3,5,3'TRIIODOTHYRONINE | C15 H12 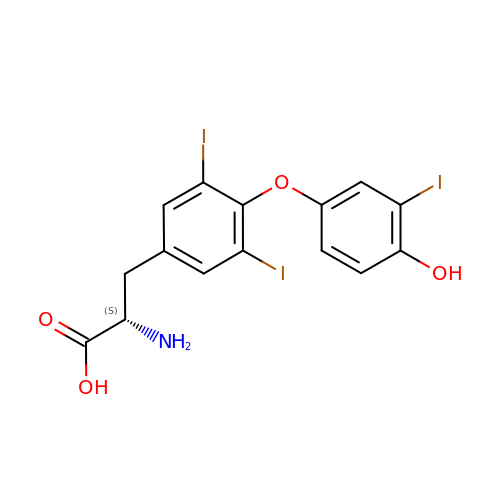I3 N O4 | AUYYCJSJGJYCDS-LBPRGKRZSA-N Paroxetine | C19 H20 F N O3 | 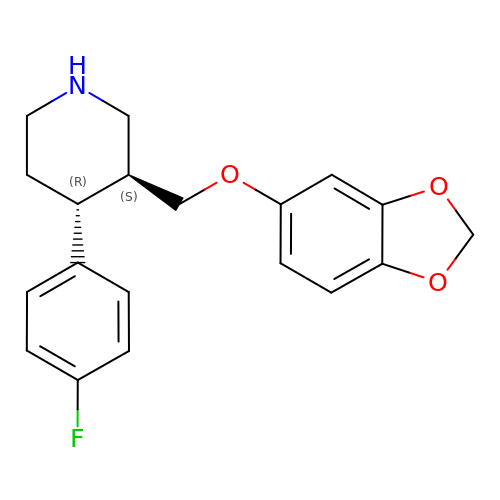AHOUBRCZNHFOSL-YOEHRIQHSA-N>DVREDRVVTNSTGNPINEPFVTQRIGEHGPLLLQDYNLIDSLAHFNRENIPQRNPHAHGSGAFGYFEVTDDITDICGSAMFSKIGKRTKCLTRFSTVGGDKGSADTVRDPRGFATKFYTEEGNLDWVYNNTPVFFIRDPSKFPHFIHTQKRNPQTNLRDADMFWDFLTTPENQVAIHQVMILFSDRGTPANYRSMHGYSGHTYKWSNKNGDWHYVQVHIKTDQGIKNLTIEEATKIAGSNPDYCQQDLFEAIQNGNYPSWTVYIQTMTERDAKKLPFSVFDLTKVWPQGQFPLRRVGKIVLNENPLNFFAQVEQAAFAPSTTVPYQEASADPVLQARLFSYADAHRYRLGPNFHQIPVNCPYASKFFN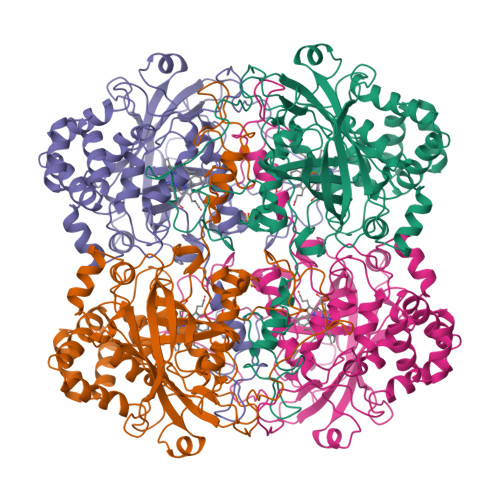PAIRDGPMNVNGNFGSEPTYLANDKSYTYIQQDRPIQQHQEVWNGPAIPYHWATSPGDVDFVQARNLYRVLGKQPGQQKNLAYNIGIHVEGACPQIQQRVYDMFARVDKGLSEAIKKVAE[4x]> MTQVLVMPKAVFESYKTAGVQFNKLLDTNYIVSETSVNDLAEIHQALTAFPFLLPEKLDIKLAVSPIIKVAELGEIDGPEQFKMKDLHNRLESRLATNELRDAGNRNLVYD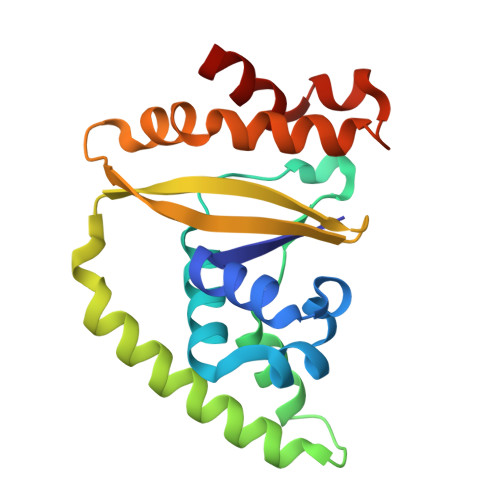YYLYPVDENLWVAVQQSAHIASSDPRRVSIQLNHTFFDSMINEMLNTRPRESVASTQIFTYYLESC> MAPKKVLLALTSYNDVFYSDGAKTGVFVVEALHPFNTFRKEGFEVDFVSETGKFGWDEHSLAKDFLNGQDETDFKNKDSDFNKTLAKIKTPKEVNADDYQIFFASAGHGTLFDYPKAKDLQDIASEIYANGGVVAAVCHGPAIFDGLTDKKTGRPLIEGKSITGFTDVGETILGVDSILKAKNLATVEDVAKKYGAK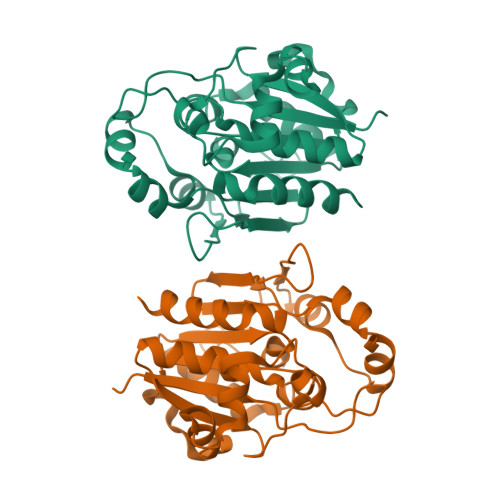YLAPVGPWDDYSITDGRLVTGVNPASAHSTAVRSIVALKNLEHHHHHH>ATRTRGYVTTKDGIKWYYEQEGSGPDVVLIPDGLGECQMFDKPMSLIASNGFRVTTFDMPGMSRSSDAPPETYQDITGRKLAGYIITLLDTLDIKIASVWGCASGASTVLALCSDYPERVRNGMPHEVPTENPDILLHIHEVDPATISQEMAANSRAASGNVEAWDALGPEVHARLHDNYPRWAYGYPRTIPP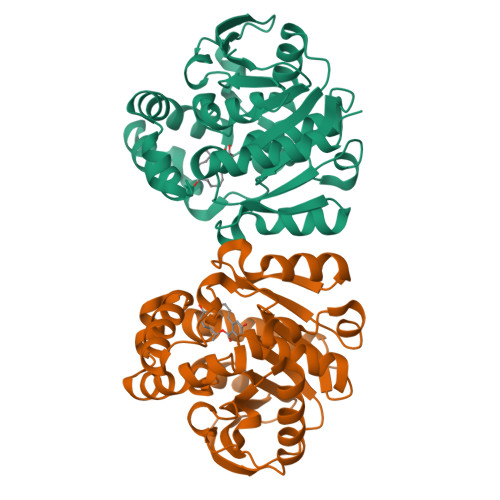SAPVKTEDLHKVPIDWTVGASTPTKLFFENIVIAAREGINIGTLPGNHFPYVSHPEEFAKYVVETSRKYLK[8x]>ASHANINAFKEAVTKIDRVEINRRLELAYAYNASIAGAKTNGEYPALKDPYSAEQKQAGVVEYARMLEVKEQIGHVIIPRINQDIPIYAGSAEENLQRGVGHLEGTSLPVGGESTHAVLTAHRGLPTAKLFTNLDKVTVGDRFYIEHIGGKIAYQVDQIKVIAPDQLEDLYVIQGEDHVTLL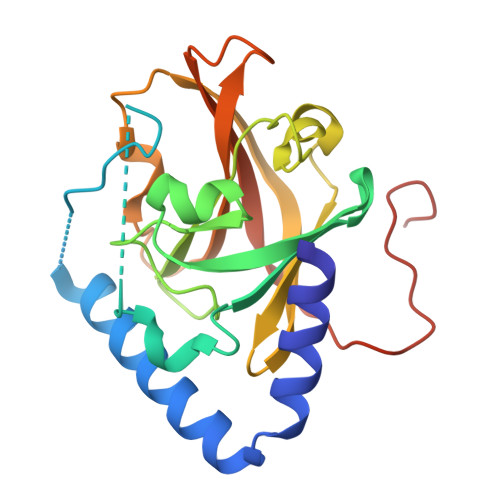TCTPYMINSHRLLVRGKRIPYVEKTVQKDSKTFRQQQYLT[2x]5-CHLORO-N-{(3S)-1-[(1S)-1-METHYL-2-MORPHOLIN-4-YL-2-5-CHLORO-N-{(3S)-1-[(1S)-1-METHYL-2-MORPHOLIN-4-YL-2-SULFONAMIDE | C19 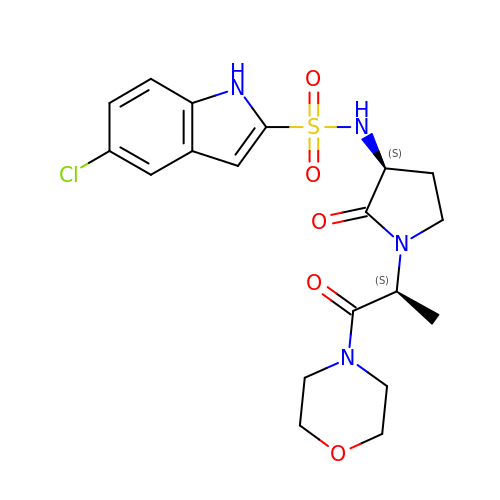H23 Cl N4 O5 S | BHNMMFGOJRIAEZ-LRDDRELGSA-N>TPATGSAEWVIPTVNAKPGEKVTMDVVVKNSAIEVAGAQFNIKQTAPIAYGSAASGDAYAAIVPNETEQYYAFGEGIGKG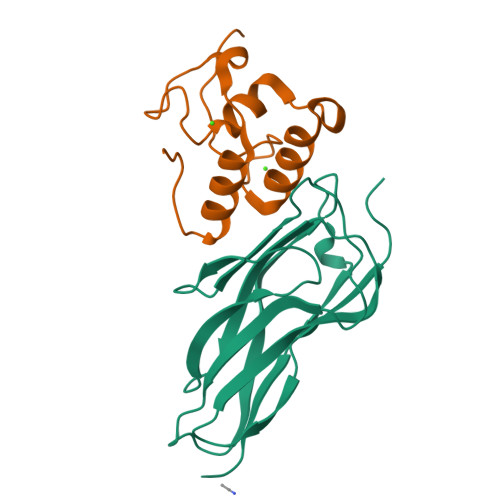IKAADGAKIITLTFNVPADCAKGTYPVKWSNAFITDTNGNKITDKITLTDGAIVVGDT[2x];>[2x]HMASKPVWGDVNCDGDVNVADVVLLNKWLNNNADYAMTDQGKVNADCFNPQDANGGAVDASKVDLTKTDSDAIIKSVVHLITLPAKG>MAKKTSSVLYGRRTRRRNEPPLDKGMIPWLGHALEFGKDAAKFLTRMKEKHGDIFTVRAAGLYITVLLDSNCYDAVLSDVASLDQTSYAQVLMKRIFNMILPSHNPESEKKRAEMHFQGASLTQLSNSMQNNLRLLMTPSEMGLKTSEWKKDGLFNLCYSLLFKTGYLTVFGAENNNSAALTQIYEEFRRFDKLLPKLARTTVNKEEKQIASAAREKLWKWLTPSGLDRKPREQSWLGSYVKQLQDEGIDAEMQRRAMLLQLWVTQGNAGPAAFWVMGYLLTHPEALRAVREEIQGGKHLRLEERQKNTPVFDSVLWETLRLTAAALITRDVTQDKKICLSNGQEYHLRRGDRLCVFPFISPQMDPQIHQQPEMFQFDRFLNADRTEKKDFFKNGARVKYPS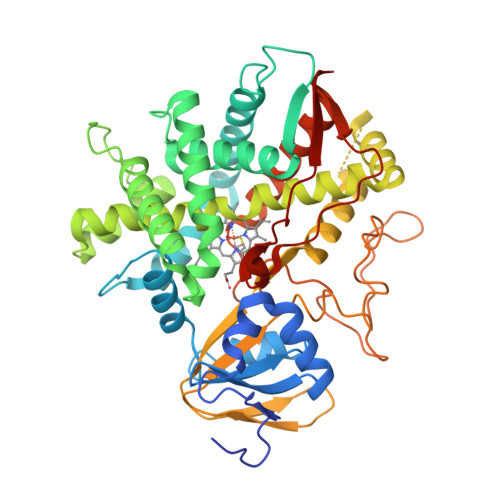VPWGTEDNLCPGRHFAVHAIKELVFTILTRFDVELCDKNATVPLVDPSRYGFGILQPAGDLEIRYRIRFHHHH[2x]> GGLGPSDRQLLLFYLEQAEANLTTLTDAVDAFFTAVATNQPPKIFVAHSKFVILSAHKLVFIGDTLSRQAKAADVRSQVTHYSNLLSDLLRG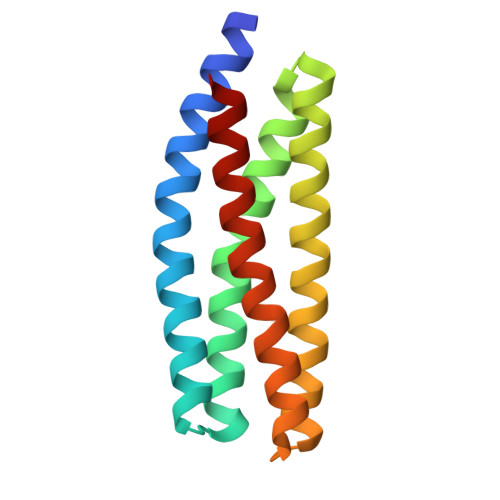IVATTKAAALQYPSPSAAQDMVDRVKELGHSTQQFRRVLGQLAAA>[2x]MILSDKDIIDYVTSKRIIIKPFNKDFVGPCSYDVTLGDEFIIYDDEVYDLSKELNYKRIKIKNSILVCPLNYNLTEEKINYF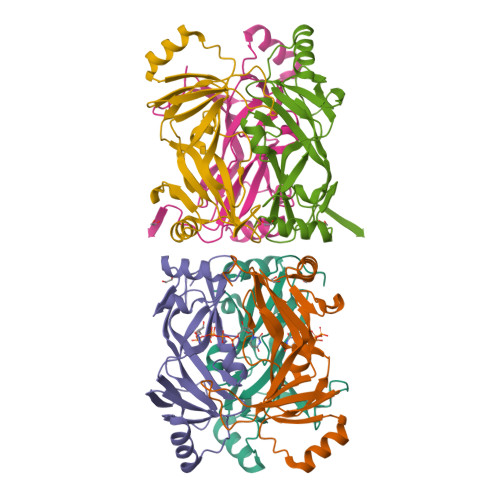KEKYNVDYVVEGGVLGTTNEYIELPNDISAQYQGRSSLGRVFLTSHQTAGWIDAGFKGKITLEIVAFDKPVILYKNQRIGQLIFSKLLSPADVGYSERKTSKYAYQKSVMPSLIHLDNHKKD> MHAAKRRNCFPGDTRILVQINGTPQRVTLKELYELFDEEHYESMVYVRKKPKVDIKVYSFNPEEGKVVLTDIEEVIKAPATDHLIRFELELGSSFETTVDHP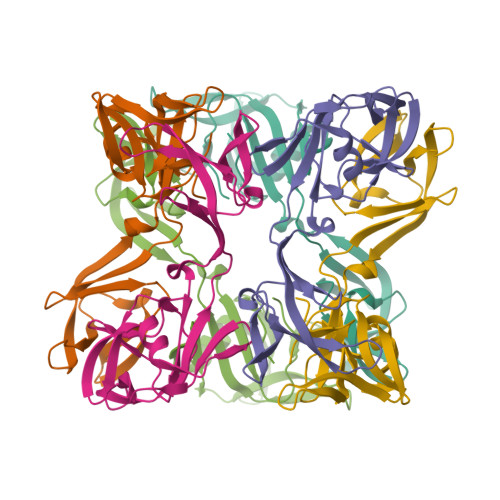VLVYENGKFVEKRAFEVREGNIIIIIDESTLEPLKVAVKKIEFIEPPEDFVFSLNAKKYHTVIINENIVTHQCDGDEDHHHHHH>MKKEFSAGGVLFKDGEVLLIKTPSNVWSFPKGNIEPGEKPEETAVR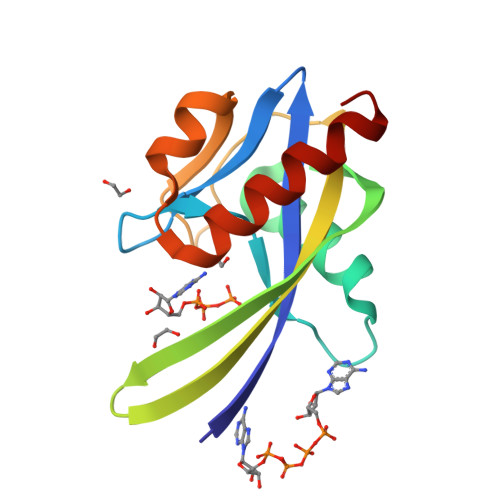EVWEETGVKGEILDYIGEIHYWYTLKGERIFKTVKYYLMKYKEGEPRPSWEVKDAKFFPIKEAKKLLKYKGDKEIFEKALKLKEKFKL[2x]>GIIETPRGAIKVTAQPTDHVVGEYLVLSPQTVLRSQKLSLIHALAEQVKTCTHNGRAGRYAVEAYDGRVLVPSGYAISPEDFQSLSESATMVYNEREFVNRKLHHIAMHGPALNTDEESYELVRAERTEHEYVYDVDQRRCCKKEEAAGLVLVGDLTNPPYHEFAYEGLKIRPACPYKIAVIGVFGVPGSGKSAIIKNLVTRQDLVTSGKKENCQEITTDVMRQRGLEISARTVDSLLLNGCNRPVDVLYVDEAFACHSGTLLALIALVRPRQKVVLCGDPKQCGFFNMMQMKVNYNHNICTQVYHKSISRRCTLPVTAIVSSLHYEGKMRTTNEYNKPIVVDTTGSTKPDPGDLVLTCFRGWVKQLQIDYRGYEVMTAAASQGLTRKGVYAVRQKVNE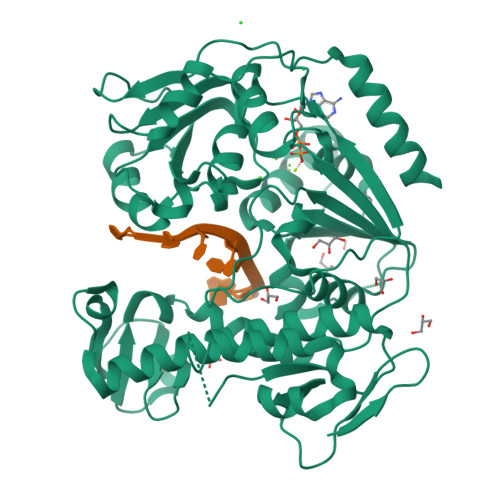NPLYASTSEHVNVLLTRTEGKLVWKTLSGDPWIKTLQNPPKGNFKATIKEWEVEHASIMAGICSHQ[2x]4,6-DIOXOHEPTANOIC ACID | C7 H10 O4 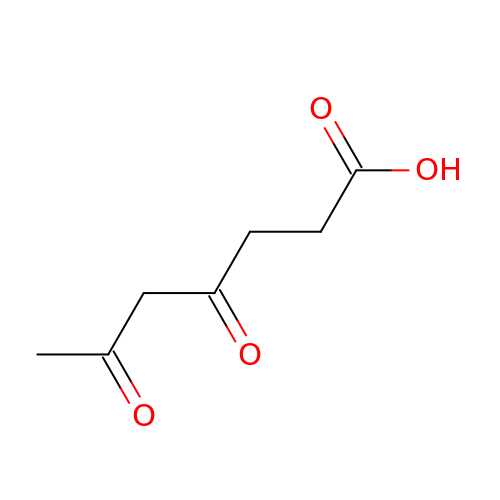| WYEPBHZLDUPIOD-UHFFFAOYSA-N> TFAYKIDGNEVIFTLWAPYQKSVKLKVLEKGLYEM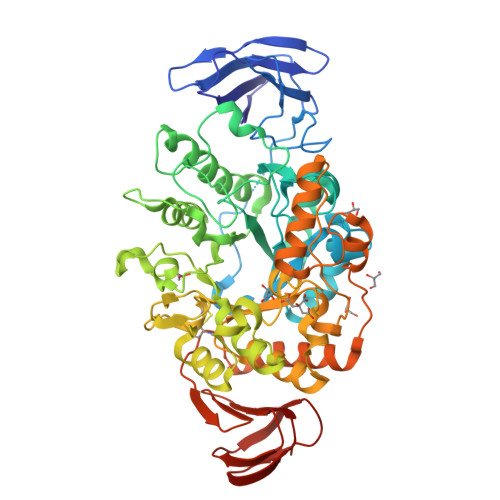ERDEKGYFTITLNNVKVRDRYKYVLDDASEIPDPASRYQPEGVHGPSQIIQESKEFNNETFLKKEDLIIYEIHVGTFTPEGTFEGVIRKLDYLKDLGITAIEIMPIAQFPGKRDWGYDGVYLYAVQNSYGGPEGFRKLVDEAHKKGLGVILDVVYNHVGPEGNYMVKLGPYFSQKYKTPWGLTFNFDDAESDEVRKFILENVEYWIKEYNVDGFRLEAVHAIIDTSPKHILEEIADVVHKYNRIVIAESDLNDPRVVNPKEKCGYNIDAQWVDDFHHSIHAYLTGERQGYYTDFGNLDDIVKSYKDVFVYDGKYSNFRRKTHGEPVGELDGCNFVVYIQNHDQVGNRGKGERIIKLVDRESYKIAAALYLLSPYIPMIFMGEEYGEENPFYFFSDFSDSKLIQGVREGRKKENGQDTDPQDESTFNASKLSWKIDEEIFSFYKILIKMRKELSIACDRRVNVVNGENWLIIKGREYFSLYVFSKSSIEVKYSGTLLLSSNNSFPQHIEEGKYEFDKGFALYKL>ALVAEDAPVLSKAFVDRVNRLNRGIWKAKYDGVMQNITLREAKRLNGVIKKNNNASILPKRRFTEEEARAPLPSSFDSAEAWPNCPTIPQIADQSACGSCWAVAAASAMSDRFCTMGGVQDVHISAGDLLACCSDCGDGCNGGDPDRAWAYFSSTGLVSDYCQPYPFPHCSHHSKSKNGYPPCSQFNFDTPKCDYTCDDPTIPVVNYRSWTSYALQGEDDYMRELFFRGPFEVAFDVYEDFIAYNSGVYHHVSGQYLGGHAVRLVGWGTSNGVPYWKIANSWNTEWGMDGYFLIRRGSSECGIEDGGSAGIPLAPNTAHHHHHHH[2x]

Bloodstream T. brucei parasites express two papain family cysteine proteases, rhodesain (brucipain, trypanopain), a cathepsin L-like enzyme and TbCatB, a cathepsin B-like enzyme. RNA interference of TbCatB is able to rescue mice from a lethal T. brucei infection. TbCatB may therefore represent the more promising target for novel cysteine protease inhibitors targeting T. brucei infection. TbCatB has an ‘occluding loop’, a unique feature of cathepsin B-like enzymes, which spans the prime side of the substrate binding site and distinguishes them from the cathepsin L-like enzymes.

The TbCatB•CA074 complex crystallized in spacegroup P21 with two molecules in the asymmetric unit and was refined to 1.60Å resolution to a final Rfree of 17.8% and Rfactor of 14.7%. Chains A and B comprise residues 78–335 and 78–337 of full-length TbCatB, respectively. With the predicted maturation cleavage site of the enzyme between Pro93 and Leu94, we were surprised to observe that our crystal structure of the activated, mature form of TbCatB contains an additional 16 residues at the N-terminus preceding the predicted site of activation. Furthermore, the extension in TbCatB establishes several polar and hydrophobic interactions with the L and R domains of the main α/β fold, as is observed in structures of FP-2 and FP-3 (although this results in the malarial extensions adopting more extended secondary structure). While a number of hydrogen bonds are formed between residues lining the substrate-binding site and the inhibitor backbone, a number of hydrophobic residues also provide binding energy, principally in the S2 subsite, the subsite that confers selectivity for this class of enzyme. This is in contrast with the TbCatB•CA074 complex where hydrogen bonding between the enzyme and inhibitor dominate over hydrophobic interactions. TbCatB has a Gly at this position, which opens up the pocket allowing larger P2 substituents to be targeted to this part of the active site cleft. In our structure Asp258175 and Asp327244 are available for binding and in each copy of TbCatB interact with a glycerol molecule from the cryoprotectant solution. In TbCatB, the loop is three residues longer than in mammalian homologs and we note a dual peptide conformation between His 194110 and His195111. The corresponding motif in TbCatB, “FNFD”, lacks this flexibility and both Phe208121 and Phe210123 stack with the N-terminal residue (Phe189105) of the occluding loop, creating a more stable opening around S1′.> SNAMESPLGSDLARLVRIWRALIDHRLKPLELTQTHWVTLHNIHQLPPDQSQIQLAKAIGIEQPSLVRTLDQLEDKGLISRQTCASDRRAKRIKLTEKAEPLIAEMEEVIHKTRGEILAGISSEEIELLIKLIA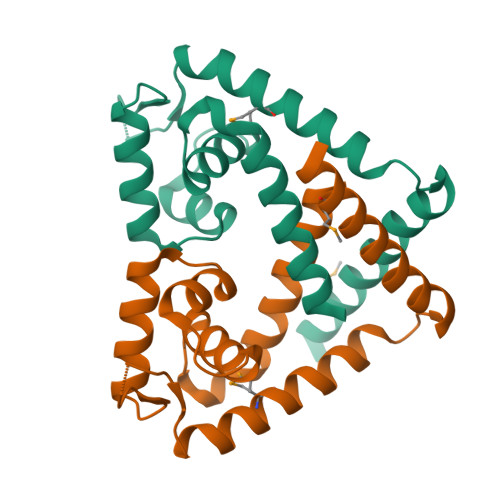KLEHNIMELHSHD> GSHMASMTGGQQMGRDPLKNVPPLTANQKSLIARLVYYQEGYEQPSEEDLKRVTQTWQSDEDDEDSDMPFRQITEMTILTVQLIVEFAKGLPGFSKISQSDQITLLKACSSEVMMLRVARRYDAATDSVLFANNQAYTRDNYRKAGMAYVIEDLLHFCRCMYSMM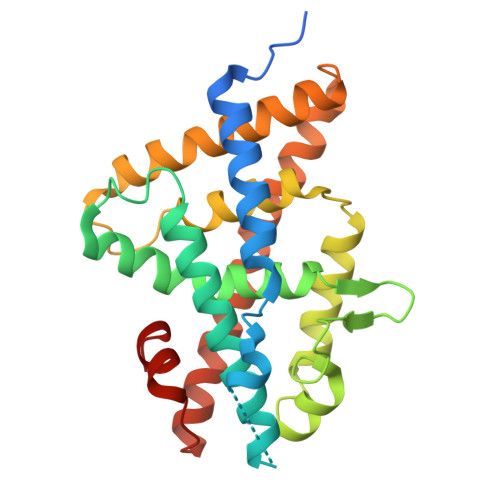MDNVHYALLTAIVIFSDRPGLEQPSLVEEIQRYYLNTLRVYILNQNSASPRSAVIFGKILGILTEIRTLGMQNSNMCISLKLKNRKLPPFLEEIWDVADVA>[14x]ALVPMVIEQTSRGERSFDIYSRLLKERVIFLTGQVEDHMANLIVAQMLF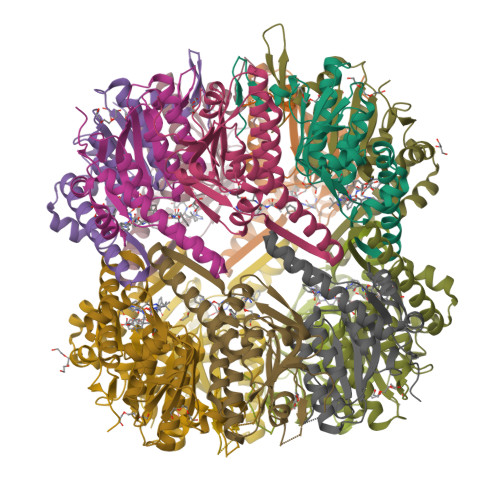LEAENPEKDIYLYINSPGGVITAGMSIYDTMQFIKPDVSTICMGQAASMGAFLLTAGAKGKRFCLPNSRVMIHQPLGGYQGQATDIEIHAREILKVKGRMNELMALHTGQSLEQIERDTERDRFLSAPEAVEYGLVDSILTHRN>[2x]MSLTNDERIL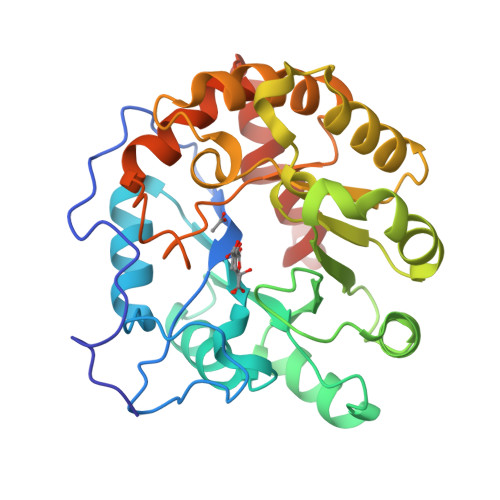SWNETPSKPRYTPPPGAIDAHCHVFGPMAQFPFSPKAKYLPRDAGPDMLFALRDHLGFARNVIVQASCHGTDNAATLDAIARAQGKARGIAVVDPAIDEAELAALHEGGMRGIRFNFLKRLVDDAPKDKFLEVAGRLPAGWHVVIYFEADILEELRPFMDAIPVPIVIDHMGRPDVRQGPDGADMKAFRRLLDSREDIWFKATCPDRLDPAGPPWDDFARSVAPLVADYADRVIWGTAWPHPNMQDAIPDDGLVVDMIPRIAPTPELQHKMLVTNPMRLYWSEEMEGHHHHHH>HVLKTKDVDTVFVERQKKVLSLFQDVDQLNTNDEYYKIGKDYDIEANIDNYTNKKAVEDFLKMYRCGFLPKYNEFSVFHDKLRDEAIALFHLFYYAKDFDTFYKSAAFARVHLNQGQFLYAYYIAIIQRKDTYGIVLPAPYEIYPELFVNIDTTYKMFRTKMQNGLINPEAAVEYGIVKEDNHYVYYSNYSNAITYYNEEQRLAYFTEDIGLNAYYFFFHIHLPFWWTAEKYGNLKERRGEMYHYFYDQLLTRYYFERLTNGLGTIPEFSWYSPVKTGHYPLLTSYYTPFSQRPNFYNVHSEENYEKIRFLDAYENYFVQALQKGVFEGFGQTIYLNDSKANSFVGNYWQDNADLYGEEVTKDYQRSYEIVARQVLGAAPKPFDKYTFMPSALDFYQTSLRDPTFYQLYNRIIGYFNQFKQYLEPHSQEKLHFVGVKVNNVVVDKLVTFFEYYDFDATNTVFLTEEELKTKYPHNLKVRQPRLNHQPFNINIDIKADVATDAVVKIFMGPKYNENGFPITLENDWMKFFEMDWFTHKITPGQNTIVRNSNEFVIFKEDSLPSTELYKLLEKGKVPFDMSEDFGYLPKRLMLPRGTKGGFPFQFVVFVYPFESTTKNLTPYEKFMIDNKPLGYPFDRPVDTSCFKQPNIFFRDVS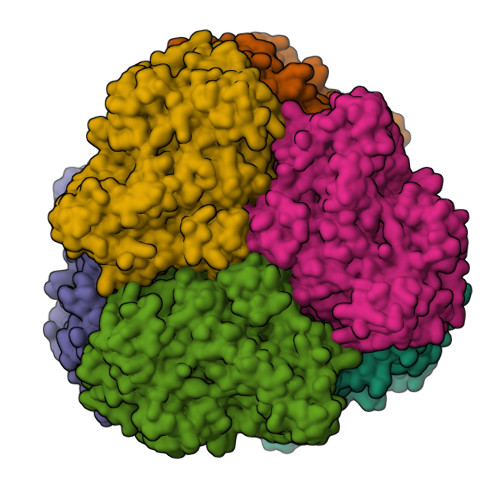VYHEGEYHAYEYNVPAYFSH[6x]> SNAIRSIWENNGFGLMSS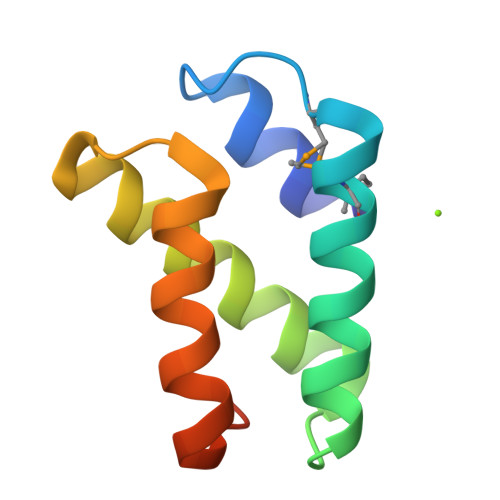KTMTDFDYWISDFEKIGASQKEAEQLIVKAIEIAIDANARNYNYINAILKDWEQRGFKSVEEREA> GHMSHLADVSPPTACRVCGGGVQEFLDLGRQPLSDRFRKPDELDDEFTYRLAVGRCDSCEMVQLTEEVPRDLMFHEVYPYHSSGSSVMREHF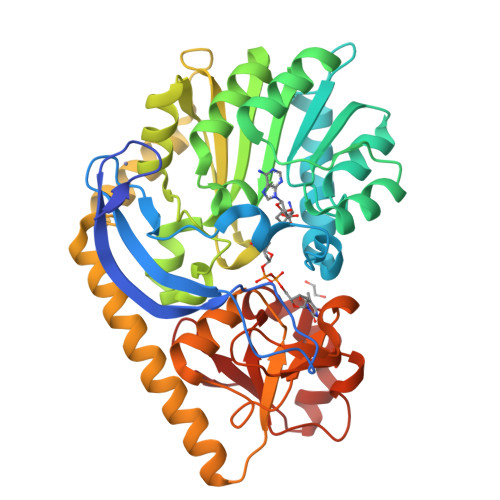AMLARDFLATELTGPDPFIVEIGCNDGIMLRTIQEAGVRHLGFEPSSGVAAKAREKGIRVRTDFFEKATADDVRRTEGPANVIYAANTLCHIPYVQSVLEGVDALLAPDGVFVFEDPYLGDIVAKTSFDQIYDENFFLFSATSVQGMAQRCGFELVDVQRLPVHGGEVRYTLARQGSRTPSAAVAQLLAAEREQELSDMATLRAFAGNVVKIRDELTALLHRLRAEGRSVVGYGATAKSATVTNFCGIGPDLVHSVYDTTPDKQNRLTPGAHIPVRPASAFSDPYPDYALLFAWNHAEEIMAKEQEFHQAGGRWILYVPEVHIR> GAMGSVSCEECGGGHSPSKLLLCDKCDRGYH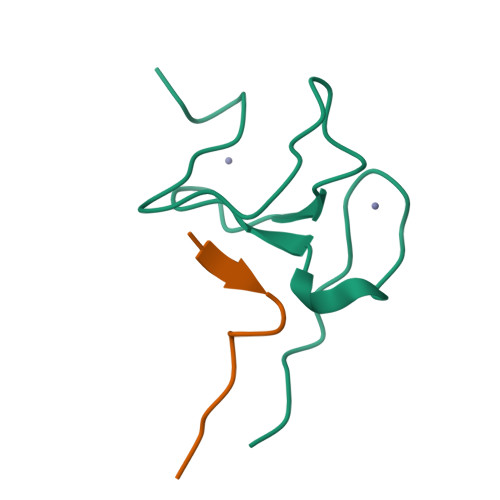LFCLRPILPSVPKGSWFCPSCSNHKPK;> ARTKQTARKSY Biotin-dependent acetyl-CoA carboxylases (ACCs) are essential enzymes that catalyse the ATP-dependent carboxylation of acetyl-CoA to malonyl-CoA. Eukaryotic ACCs, instead, are multienzymes, which integrate all functional components into a single polypeptide chain of ∼2,300 amino acids2. In addition to the canonical ACC components, eukaryotic ACCs contain two non-catalytic regions, the large central domain (CD) and the BC–CT interaction domain (BT). Here we provide the structure of Saccharomyces cerevisiae (Sce) ACC CD, intermediate- and low-resolution structures of human (Hsa) ACC CD and larger fragments of fungal ACC from Chaetomium thermophilum (Cth).

Using molecular replacement based on fungal ACC CD and CT models, we obtained structures of a variant comprising CthCT and CDC1/CDC2 in two crystal forms at resolutions of 3.6 and 4.5 Å (CthCD-CTCter1/2), respectively, as well as of a CthCT linked to the entire CD at 7.2 Å resolution (CthCD-CT). In all these crystal structures, the CT domains build a canonical head-to-tail dimer29, with active sites formed by contributions from both protomers. The connection of CD and CT is provided by a 10-residue peptide stretch, which links the N terminus of CT to the irregular β-hairpin/β-strand extension of CDC2. The connecting region is remarkably similar in isolated CD and CthCD-CTCter structures, indicating inherent conformational stability. CD/CT contacts are only formed in direct vicinity of the covalent linkage and involve the β-hairpin extension of CDC2 as well as the loop between strands β2/β3 of the CT N-lobe, which contains a conserved RxxGxN motif. The neighbouring loop on the CT side (between CT β1/β2) is displaced by 2.5 Å compared to isolated CT structures. On the basis of an interface area of ∼600 Å2 and its edge-to-edge connection characteristics, the interface between CT and CD might be classified as conformationally variable. Indeed, the comparison of the positioning of eight instances of the C-terminal part of CD relative to CT in crystal structures determined here, reveals flexible interdomain linking. The CDC2/CT interface acts as a true hinge with observed rotation up to 16°, which results in a translocation of the distal end of CDC2 by 8 Å.

>[2x]GNLREVRYHDEERPYFIDWDFALRKSGANQTESSMHMQSVVPSSPATPVENDFKRIHSISDMTYLARRTRDEPIRKGVIVPCKDLLDAEEALSRALEVLPLAHKETKDKDRKQQPGIAADLAQRRRPGTPLRLEGIGELSAVVNVAVRDAEGKNDEEILALIKPWVQNSKADLLARRVRRLTFICGRNDGSYPSYYTFRGPDYAEDDSIRHIEPSLAFQLELGRLSKFKLTPVFTQNKNIHVYEAVGRGVETDRRYFTRAVVRPGRLRDEISTAEYLISEADRVVNDIFDALEIIGTNKTDLNHMFINFSHTFQVTADEVAESLQGFLDRFGPRGWRLRVHQVEIRINCMRSDNNDENDTMPLRVIITNTSGFVIQIELYEEKLSEKGEWVYYYVSGNAKIGSMHLLPVSTPYPTKNWLQPKRYKAHILGTQYVYDFPELFRQAIQNSWTEAVKKIPSLAAKQPAIGECIDYNELVLGDQDNLAEVSREPGMNSTGMVGWLINARTPEYPDGRKFIVVANDITFKIGSFGPKEDTFFFKCTELARKMGIPRIYLSANSGARLGLAEELMPHFNVAWNDPAKPEAGFKYLYLSDEAKRRFENEVITEEIVEDGEKRHKIITIVGAEEGLGVECLRGSGLIAGATSRAYNDIFTCTLVTCRSVGIGAYLVRLGQRAVQVEGQPIILTGAPALNSLLGREVYTSNLQLGGTQIMYRNGVSHLTAKDDFDGVTKIVQWLSFIPDQRNNPLPILSPSPDPWDRDVVYTPPYKQTYDVRWMIAGKEDEDGFQPGLFDKDSFVETLGGWARTVVVGRARLGGIPMGVIAVETRTIENITPADPANPDSIEQVTNEAGGVWYPNSAFKTAQAINDFNYGEQLPLMILANWRGFSGGQRDMYNEVLKYGSFIVDALTRFEKPIFIYIPPHGELRGGSWVVVDPTINPASMEMYADEEARGGVLEPEGIIPIKYKKDKQLETMARLDPVYRSLKKEMAKEGLSKEESDNIKKKMQQREELLLPIYHQICVQFADLHDRAGRMKAKGVIRQSLQWRQSRRFFYWRVRRRLIEDDILRRIEEAINPAGKRRHDPENTSLAASPETRSPHLVQLESWVGIPGFKTNDREVVEWYEQNQDRINEKLEKLKKESIADQMRELLRAAEXXXXXXXXXXXXXXXXXXXXXXXXXXX> MVEATAQETDRPRFSFSIAAREGKARTGTIEMKRGVIRTPAFMPVGTAATVKALKPETVRATGADIILGNTYHLMLRPGAERIAKLGGLHSFMGWDRPILTNSGGYQVMSLSSLTKQSEEGVTFKSHLDGSRHMLSPERSIEIQHLLGSDIVMAFDECTPYPATPSRAASSMERSMRWAKRSRDAFDSRKEQAENAALFGIQQGSVFENLRQQSADALAEIGFDGYAVGGLAVGEGQDEMFRVLDFSVPML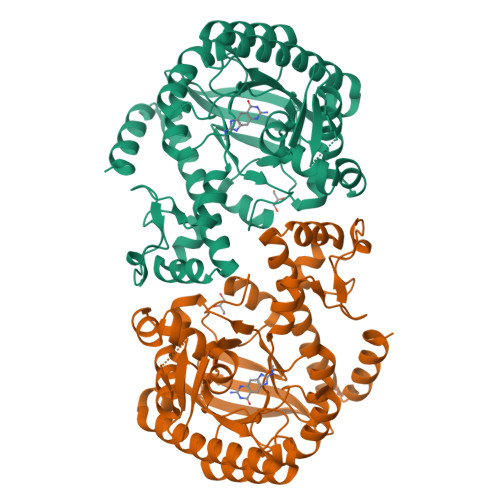PDDKPHYLMGVGKPDDIVGAVERGIDMFDCVLPTRSGRNGQAFTWDGPINIRNARFSEDLKPLDSECHCAVCQKWSRAYIHHLIRAGEILGAMLMTEHNIAFYQQLMQKIRDSISEGRFSQFAQDFRARYFARNS N-({2-[8-(2-methoxyethoxy)naphthalen-2-yl]-1,3-thiazol-4-yl}acetyl)glycine | C20 H20 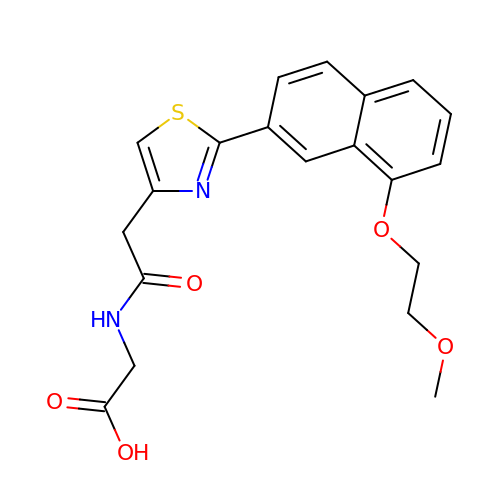N2 O5 S | XOTNABKQGYEPBQ-UHFFFAOYSA-N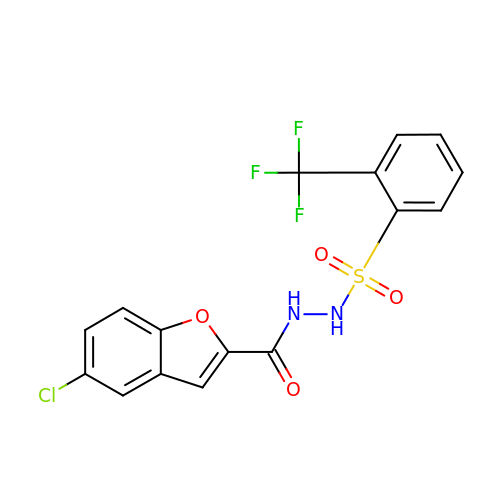N'-(5-CHLOROBENZOFURAN-2-CARBONYL)-2-(TRIFLUOROMETHYL)BENZENESULFONOHYDRAZIDE | C16 H10 Cl F3 N2 O4 S | ZLQBZYKAQQWOTK-UHFFFAOYSA-N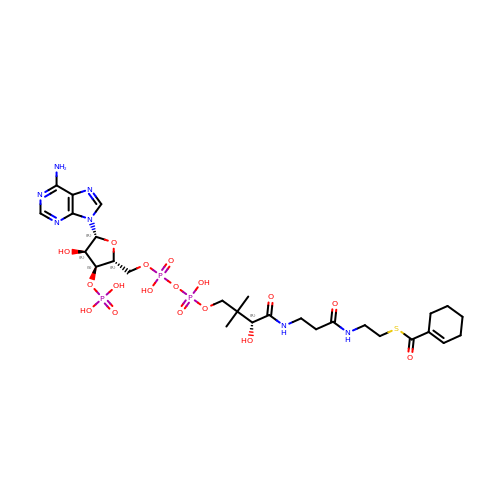1-monoenoyl-CoA | C28 H44 N7 O17 P3 S | YTTZSBMCHSFQSJ-TYHXJLICSA-N> GVAL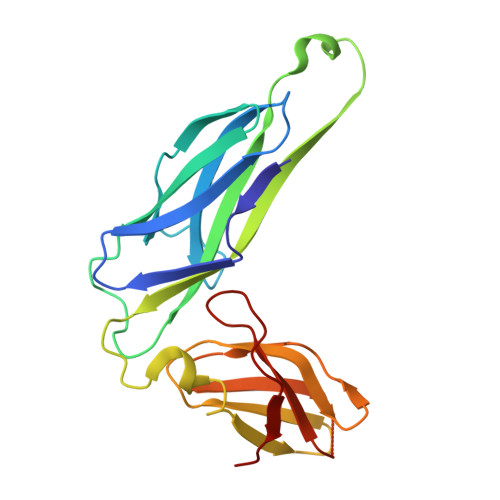GATRVIYPAGQKQVQLAVTNNDENSTYLIQSWVENADGVKDGRFIVTPPLFAMKGKKENTLRILDATNNQLPQDRESLFWMNVKAIPSMDKSKLTENTLQLAIISRIKLYYRPAKLALPPDQAAEKLRFRRSANSLTLINPTPYYLTVTELNAGTRVLENALVPPMGESAVKLPSDAGSNITYRTINDYGALTPKMTGVME> GSSVTVHSSEPEVRIPENNPVKLSCA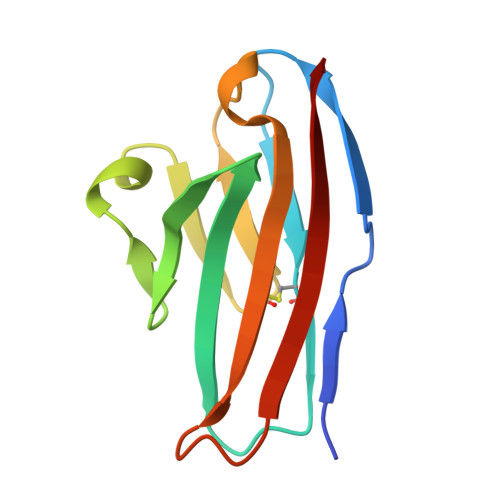YSGFSSPRVEWKFDQGDTTRLVCYNNKITASYEDRVTFLPTGITFKSVTREDTGTYTCMVSEEGGNSYGEVKVKLIVL> DHPFTEIKSGFLERRSKFLKSYSKGYYVLTPNFLHEFKTADRKKDLVPVMSLALSECTVTEHSRKNSTSSPNSTGSDAKFVLHAKQNGIIRRGHNWVFKADSYESMMSWFDNLKILTSTS;> DHPFTEIKSGFLERRSKFLKSYSKGYYVLTPNFLHEFKTADRKKDLVPVMSLALSECTVTEHSRKNSTS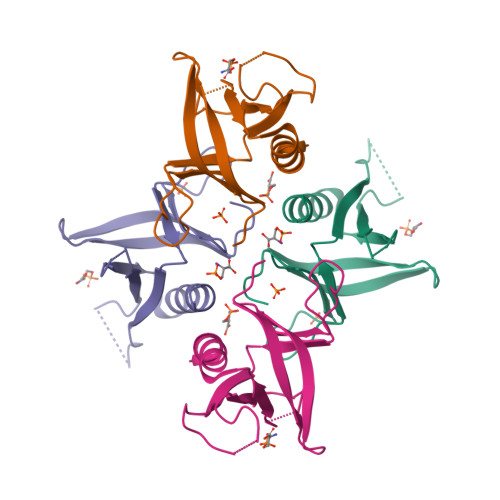SPNSTGSDAKFVLHAKQNGIIRRGHNYVFKADSYESMMSWFDNLKILTSTS> EFRCSSDAPPPAPVGDDLTEPKELTDLFEKAKKAVIDRLHEDEKALRARGEAPRCTADKLIFRREYGSLSKDERLAYVNAVKCLQSKPPRTPASVAPGARSRFDDFVVVHIQQTLDIHYSGIFQAWHRWFVYQYEKALRDECGYTGYQPYWDWPKYASAPQDSPLFNGDPYSLGGNGEYVPHDGPVIVPPEGVSGGNISLPAGVGGGFVRTGPFANMTVNLGPVGGLADTAPGPQGGLGYNPRGLKRDLGGAMNTRYANYTTVLRLLTQPDVDAFRTVSEGVPYTVEIGPHNGIHYTIGGDPGGDLFTSPGDPAFW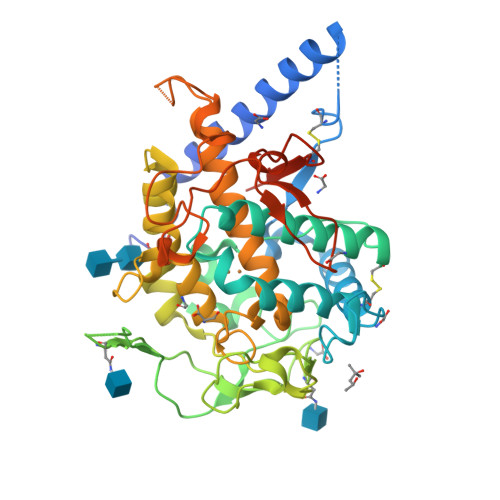VHHAQMDRVWATWQALGLLPPADGGDPDPARRYTDLGKGDYAHRTWQNSPPSPFAELSDVIDMGYAAPSTTIGAVMSTTEGELCYFYLEQKLISEEDLNSAVDHHHHHH>[2x]QNRTVKGTVISSEDNEPLIGANVVVVGNTTIGAATDLDGNFTLSVPANAKMLRVSYSGMTTKEVAIANVMKIVLDPDSKVLEQVVVLGYGTGQKLSTVSGSVAKVSSEKLAEKPVANIMDALQGQVAGMQVMTTSGDPTAVASVEIHGTGSLGASSAPLYIVDGMQTSLDVVATMNPNDFESMSVLKDASATSIYGARAANGVVFIQTKKGKMSERGRITFNASYGISQILNTKPLDNMMTGDELLDFQVKAGFWGNNQTVQKVKDMILAGAEDLYGNYDSLKDEYGKTLFPVDFNHDADWLKALFKTAPTSQGDISFSGGSQGTSYYASIGYFDQEGMAREPANFKRYSGRLNFESRINEWLKVGANLSGAIANRRSADYFGKYYMGSGTFGVLTMPRYYNPFDVNGDLADVYYMYGATRPSMTEPYFAKMRPFSSESHQANVNGFAQITPIKGLTLKAQAGVDITNTRTSSKRMPNNPYDSTPLGERRERAYRDVSKSFTNTAEYKFSIDEKHDLTALMGHEYIEYEGDVIGASSKGFESDKLMLLSQGKTGNSLSLPEHRVAEYAYLSFFSR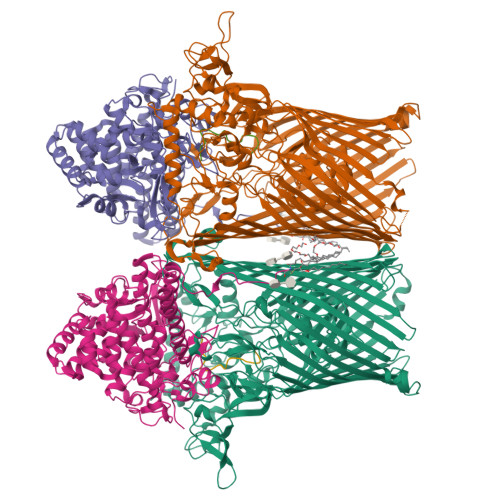FNYGFDKWMYIDFSVRNDQSSRFGSNNRSAWFYSVGGMFDIYNKFIQESNWLSDLRLKMSYGTTGNSEIGNYNHQALVTVNNYTEDAMGLSISTAGNPDLSWEKQSQFNFGLAAGAFNNRLSAEVDFYVRTTNDMLIDVPMPYISGFFSQYQNVGSMKNTGVDLSLKGTIYQNKDWNVYASANFNYNRQEITKLFFGLNKYMLPNTGTIWEIGYPNSFYMAEYAGIDKKTGKQLWYVPGQVDADGNKVTTSQYSADLETRIDKSVTPPITGGFSLGASWKGLSLDADFAYIVGKWMINNDRYFTENGGGLMQLNKDKMLLNAWTEDNKETDVPKLGQSPQFDTHLLENASFLRLKNLKLTYVLPNSLFAGQNVIGGARVYLMARNLLTVTKYKGFDPEAGGNVGKNQYPNSKQYVAGIQLSF;>[2x]CELDRDPEGKDFQQPYTSFVQTKQNRDGLYALLRNTENPRMHFYQELQSDMYCTTITDGNSLAPFVNWDLGILNDHGRADEDEVSGIAGYYFVYNRLNQQANAFVNNTEAALQNQVYKNSTEIANAKSFLAEGKVLQALAIWRLMDRFSFHESVTEVNSGAKDLGVILLKEYNPGYIGPRATKAQCYDYILSRLSEAIEVLPENRESVLYVSRDYAYALRARIYLALGEYGKAAADAKMVVDKYPLIGAADASEFENIYRSDANNPEIIFRGFASATLGSFTATTLNGAAPAGKDIKYNPSAVPFQWVVDLYENEDFRKSVYIAKVVKKDKGYLVNKFLEDKAYRDVQDKPNLKVGARYFSVAEVYLILVESALQTGDTPTAEKYLKALSKARGAEVSVVNMEALQAERTRELIGEGSRLRDMVRWSIPNNHDAFETQPGLEGFANTTPLKAQAPVGFYAYTWEFPQRDRQTNPQLIKNWPIHHHHHH;>QTAGANSQRGSAG[2x]>[8x]MERTFLMIKPDAVQRNLIGEVISRIERKGLKLVGGKLMQVPMELAETHYGEHQGKPFYNDLISFITSAPVFAMVVEGEDAVNVSRHIIGSTNPSEASPGSIRGDLGL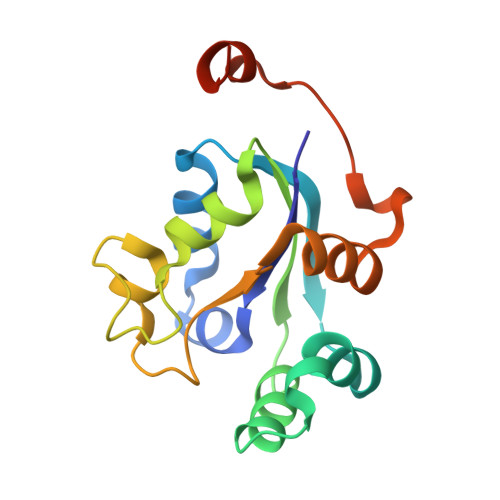TVGRNIIHGSDSLESAEREINLWFNENEITSYASPRDAWLYELEHHHHHH>QTPTGIYYEVRGDTIYMINVTSGEETPIHLFGVNWFGFETPNHVVHGLWKRNWEDMLLQIKSLGFNAIRLPFCTESVKPGTQPIGIDYSKNPDLRGLDSLQIMEKIIKKAGDLGIFVLLDYHRIGCTHIEPLWYTEDFSEEDFINTWIEVAKRFGKYWNVIGADLKNEPHSVTSPPAAYTDGTGATWGMGNPATDWNLAAERIGKAILKVAPHWLIFVEGTQFTNPKTDSSYKWGYNAWWGGNLMAVKDYPVNLPKNKLVYSPHVYGPDVYNQPYFGPAKGFPDNLPDIWYHHFGYVKLELGYSVVIGEFGGKYGHGGDPRDVIWQNKLVDWMIENKFCDFFYWSWNPDSGDTGGILQDD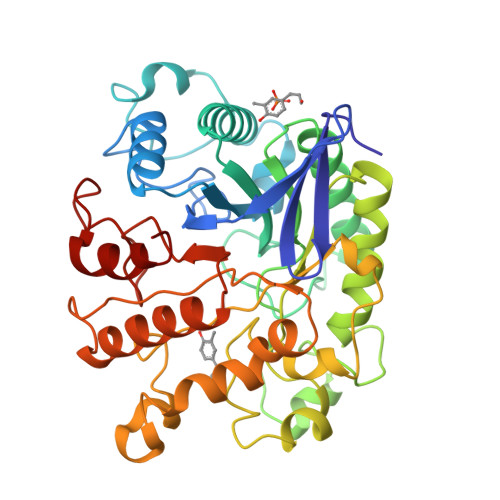WTTIWEDKYNNLKRLMD[3x]>[2x]RSSLDLQLKNARNLAGLIIHDIDGYMMKGDSSEVDRFISAVKSKNFIMDLRVFDEQAKEVSPTPSQTPNAKIQQA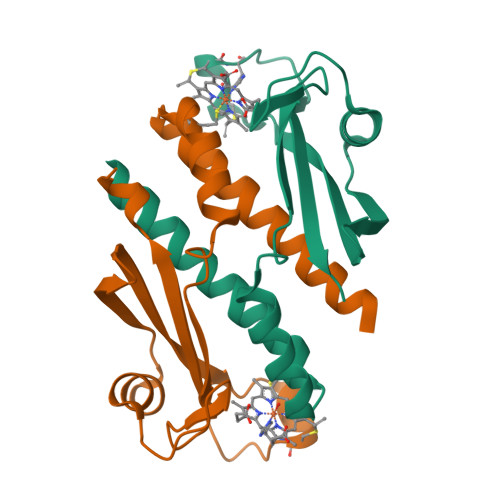IAAGRTLEFKETLDGKRTLSLVLPFPNEQRCQSCHDAGAAYLGGLLVTTSIEEGYEGARH> SGGSSSIFLLSNVSEEARQRAEEYVRRISK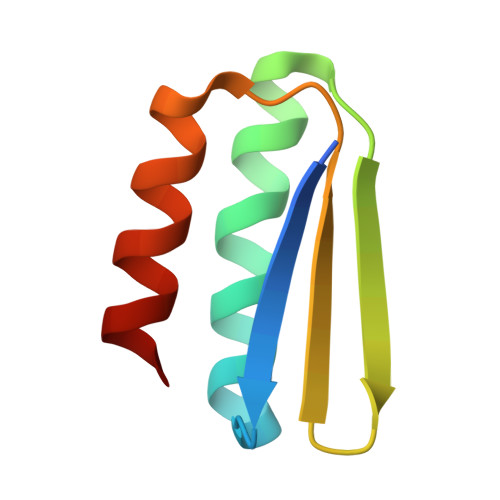KEGTEVRFEKDDGFLTIEVKNLSEERLREIAEYLWRVAV> MLSQNVAKTTVPSYYMIRTNLPHRKPQNQWEGVYYYSGITKRQRHLILLHRKREREAHMRSFNISRASVLQRLEQLSGDRKQESLPPHVRLDLAVRLAQHGLYQQATPIVDELHHQKALHAGHYALLINALACPRLGQRILHCDAQCDPALTYKLLGDENGEERAQEAYRWFDLALTSLAVDCGGRTQPSHFVPYLPQGTAAASHITNALMRTLLTCGYTHVAAIPDSVYDRMGSMGISPTISTYELVMLALSLQGNMVEAESILSFLRSHHSEHITVESFNALLLGHREARQFDCCDAIWQELVDR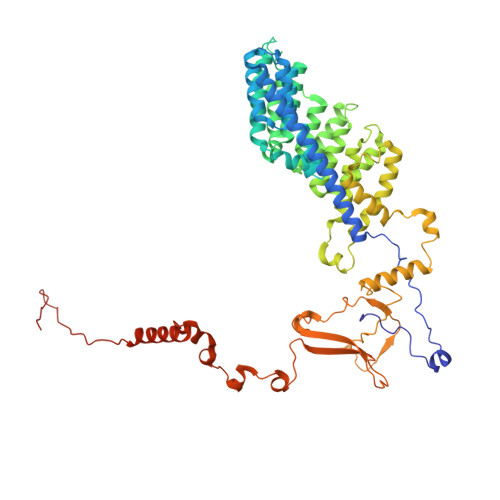RWPRASPLTAELYLRSIMDHANTPTSEPLQSFANINVVEKKKVPLVLAQMDELGVPRTHLSRVLMDEVEDSLRKFQTYRSRFYEWGRAVKQFDFIEFRRRNGWLYDLHLMKCTTKQVGPLRDFNDPDAVQGAVATAEIPAFFNERPAWERPPLEETLYVTTNKERYDDVRGGDIYYDDTRGLHDRSPTWMNEVPETRYDRLYGVNHPDIAKIGIRRHLNVEYVNRKEVVERDAALMKKTLSSGRRLRHRVESSRTHRNAGSLSGISSTAGGGSR> DYKDDDDKSLEVLFQGPMDVDAEREKITQEIKELERILDPGSSGSHVEISESSLESDSEADSLPSE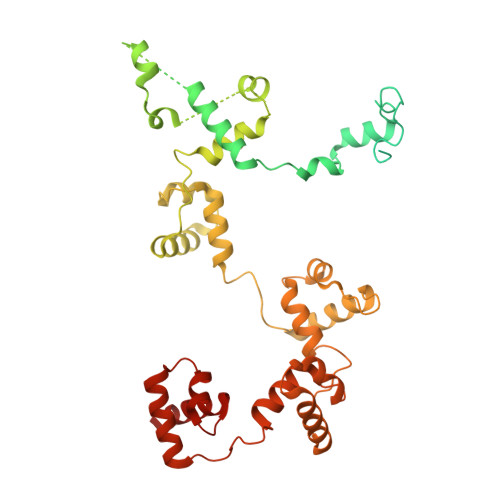DLDPADPPISEEERWGEASNDEDDPKDKTLPEDPETCLQLNMVYQEVIQEKLAEANLLLAQNREQQEELMRDLAGSKGTKVKDGKSLPPSTYMGHFMKPYFKDKVTGVGPPANEDTREKAAQGIKAFEELLVTKWKNWEKALLRKSVVSDRLQRLLQPKLLKLEYLHQKQSKVSSELERQALEKQGREAEKEIQDINQLPEEALLGNRLDSHDWEKISNINFEGSRSAEEIRKFWQNSEHPSINKQEWSREEEERLQAIAAAHGHLEWQKIAEELGTSRSAFQCLQKFQQHNKALKRKEWTEEEDRMLTQLVQEMRVGSHIPYRRIVYYMEGRDSMQLIYRWTKSLDPGLKKGYWAPEEDAKLLQAVAKYGEQDWFKIREEVPGRSDAQCRDRYLRRLHFSLKKGRWNLKEEEQLIELIEKYGVGHWAKIASELPHRSGSQCLSKWKIMMGKKQGL>[2x]YYPPALTGLRGSHPGAFEVAHQMGWEKKTFDVDHLPIEEEYDLVVVGGGISGLAAAWFYRERHPAARILVIENHDDFGGHAKRNEFQAGGRTILGYGGSESLQSPNALYSEDAKHLLKRLGVELKRFETAFDTDFYPGLGLSRAVFFDKASFGVDKLVSGDPTPMVADEVPRDRLNARSWRAFIGDFPLSREDREALIALYESPRDYLAGKSVEEKETYLAKTSYRDYLLKNVGLSETSVKYFQGRSNDFSALGADALPAADAYAAGFPGFD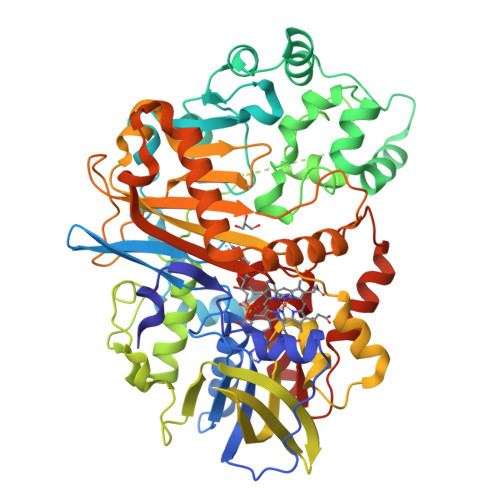ALGLPQPSEEAQAEMDEPYIYHFPDGNASLARLMVRDLIPAVAPGRGMEDIVMARFDYSKLDLAGHPVRLRLNSTAVSVRNRAGGVDVGYSRAGRLHRVRGKHCVMACYNMMVPYLLRDLSEEQAHALSQNVKFPLVYTKVLLRNWQAWKTLGIHEIYAPTLPYSRIKLDFPVDLGSYRHPRDPRQPIGVHMVYVPTTPNAGMDARTQARVGRSKLYAMSFEQLEKDIRDQLQAMLGPAGFDHRRDITGITVNRWSHGYSYFMNTLYDDEAESEALMELARSKVGNVAIANSDAAWDAYAHAAIDQAVRAVRELG(6S)-2,6-anhydro-1-deoxy-6-(2-{[(S)-hydroxy(oxido)-lambda~5~-phosphanyl]oxy}ethyl)-D-galactitol | C8 H17 O8 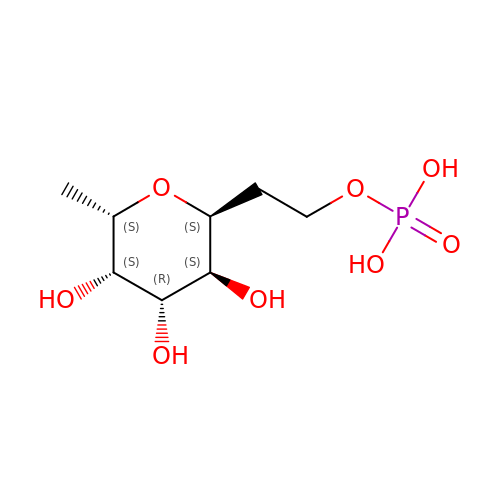P | OCKMEQYTTIUDMB-TVNFTVLESA-N> MYSVLKQSIRPRLLATHNQFRTMITAQAVLYTQHGEPKDVLFTQSFEIDDDNLAPNEVIVKTLGSPINPS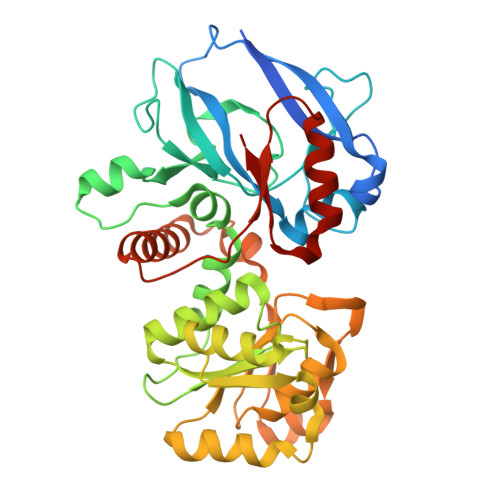DINQIQGVYPSKPAKTTGFGTAEPAAPCGNEGLFEVIKVGSNVSSLEAGDWVIPSHVNFGTWRTHALGNDDDFIKLPNPAQSKANGKPNGLTINQGATISVNPLTAYLMLTHYVKLTPGKDWFIQNGGTSAVGKYASQIGKLLNFNSISVIRDRPNLDEVVASLKELGATQVITEDQNNSKEFGPTIKEWIKQSGGEAKLALNCVGGKSSTGIARKLNNNGLMLTYGGMSFQPVTIPTSLYIFKNFTSAGFWVTELLKNNKELKTSTLNQIIAWYEEGKLTDAKSIETLYDGTKPLHELYQDGVANSKDGKQLITY> MKKEVRKVRIALASPEKIRSWSYGEVEKPETINYRTLKPERDGLFDERIFGPIKDYECACGKYKRQRFEGKVCERCGVEVTKSIVRRYRMGHIELATPAAHIWFVKDVPSKIGTLLDLSATELEQVLYFSKYIVLDPKGAILNGVPVEKRQLLTDEEYRELRYGKQETYPLPPGVDALVKDGEEVVKGQELAPGVVSRLDGVALYRFPRRVRVEYVKKERAGLRLPLAAWVEKEAYKPGEILAELPEPYLFRAEEEGVVELKELEEGAFLVLRREDEPVATYFLPVGMTPLVVHGEIVEKGQPLAEAKGLLRMPRQVRAAQVEAEEEGETVYLTLFLEWTEPKDYRVQPHMNVVVPEGARVEAGDKIVAAIDPEEEVIAEAEGVVHLHEPASILVVKARVYPFEDDVEVSTGDRVAPGDVLADGGKVKSDVYGRVEVDLVRNVVRVVESYDIDARMGAEAIQQLLKELDLEALEKELLEEMKHPSRARRAKARKRLEVVRAFLDSGNRPEWMILEAVPVLPPDLRPMVQVDGGRFATSDLNDLYRRLINRNNRLKKLLAQGAPEIIIRNEKRMLQEAVDALLDNGRRGAP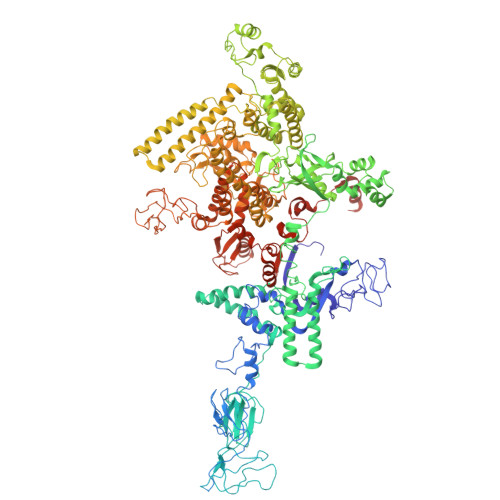VTNPGSDRPLRSLTDILSGKQGRFRQNLLGKRVDYSGRSVIVVGPQLKLHQCGLPKRMALELFKPFLLKKMEEKGIAPNVKAARRMLERQRDIKDEVWDALEEVIHGKVVLLNRAPTLHRLGIQAFQPVLVEGQSIQLHPLVCEAFNADFDGDQMAVHVPLSSFAQAEARIQMLSAHNLLSPASGEPLAKPSRDIILGLYYITQVRKEKKGAGLEFATPEEALAAHERGEVALNAPIKVAGRETSVGRLKYVFANPDEALLAVAHGIVDLQDVVTVRYMGKRLETSPGRILFARIVAEAVEDEKVAWELIQLDVPQEKNSLKDLVYQAFLRLGMEKTARLLDALKYYGFTFSTTSGITIGIDDAVIPEEKKQYLEEADRKLLQIEQAYEMGFLTDRERYDQILQLWTETTEKVTQAVFKNFEENYPFNPLYVMAQSGARGNPQQIRQLCGLRGLMQKPSGETFEVPVRSSFREGLTVLEYFISSHGARKGGADTALRTADSGYLTRKLVDVTHEIVVREADCGTTNYISVPLFQPDEVTRSLRLRKRADIEAGLYGRVLAREVEVLGVRLEEGRYLSMDDVHLLIKAAEAGEIQEVPVRSPLTCQTRYGVCQKCYGYDLSMARPVSIGEAVGIVAAQSIGEPGTQLTMRTFHTGGVAGAADITQGLPRVIELFEARRPKAKAVISEIDGVVRIEETEEKLSVFVESEGFSKEYKLPKEARLLVKDGDYVEAGQPLTRGAIDPHQLLEAKGPEAVERYLVEEIQKVYRAQGVKLHDKHIEIVVRQMMKYVEVTDPGDSRLLEGQVLEKWDVEALNERLIAEGKTPVAWKPLLMGVTKSALSTKSWLSAASFQNTTHVLTEAAIAGKKDELIGLKENVILGRLIPAGTGSDFVRFTQVVDQKTLKAIEEARKEAVEAKERPAARRGVKREQPGKQAHHHHHHHHHH The combined data indicate that 7947882 and 7904688 are prodrugs activated by the EthA monooxygenase, which then target PyrG, a cytidine triphosphate (CTP) synthetase catalyzing the ATP-dependent amination of uridine triphosphate (UTP) to form the essential pyrimidine nucleotide CTP. The crystal structure of PyrG was solved by molecular replacement on a 2.0-Å resolution data set. This structure showed a bidomain enzyme with an N-terminal amidoligase (ALase) domain, also commonly known as the synthetase domain (residues 1–278), connected through an interdomain linker (residues 279–Pro298) to a C-terminal glutamine amidotransferase (GATase) domain (residues 299–552), both domains displaying a Rossmann-like fold. On the other hand, the 34-residue C-terminal extension of M. tuberculosis PyrG, which has no predicted secondary structure or known function, could not be traced due to the lack of supporting electron density, suggesting a high degree of flexibility.

The enzyme, in complex with either UTP, at 2.0-Å resolution, or UTP plus the non-hydrolyzable ATP analog AMP-PCP and the glutamine analog 5-oxo-L-norleucine (3.5 Å), is a homotetramer with crystallographic 222 symmetry, consistent with previous studies reporting positive cooperativity for ATP and UTP due to nucleotide-driven tetramerization. Also, consistent with the oligomeric assembly as a dimer of dimers being triggered by ATP/UTP, the nucleotide-binding pockets were delimited by residues from two (ATP) or three (UTP) different subunits. Surprisingly, in the highest-resolution structure available, UTP was found lying in both pockets, a likely artifact due to the high concentration of the nucleotide (5 mM) in the co-crystallization conditions. It should be noted that the UTP orientation in the substrate-binding pocket is unproductive for the course of the reaction, as the pyrimidine ring points away from ATP.

> GMRKHPQTATKHLFVSGGVASSLGKGLTASSLGQLLTARGLHVTMQKLDPYLNVDPGTMNPFQHGEVFVTEDGAETDLDVGHYERFLDRNLPGSANVTTGQVYSTVIAKERRGEYLGDTVQVIPHITDEIKRRILAMAQPDADGNRPDVVITEIGGTVGDIESQPFLEAARQVRHYLGREDVFFLHVSLVPYLAPSGELKTKPTQHSVAALRSIGITPDALILRCDRDVPEALKNKIALMCDVDIDGVISTPDAPSIYDIPKVLHREELDAFVVRRLNLPFRDVDWTEWDDLLRRVHEPHETVRIALVGKYVELSDAYLSVAEALRAGGFKHRAKVEICWVASDGCETTSGAAAALGDVHGVLIPGGFGIRGIEGKIGAIAYARARGLPVLGLCLGLQCIVIEAARSVGLTNANSAEFDPDTPDPVIATMPDQEEIVAGEADLGGTMRLGSYPAVLEPDSVVAQAYQTTQVSERHRHRYEVNNAYRDKIAESGLRFSGTSPDGHLVEFVEYPPDRHPFVVGTQAHPELKSRPTRPHPLFVAFVGAAIDYKAGELLPVEIPEIPEHTPNGSSHRDGVGQPLPEPASRG> GPTGEAVERAIARVADTIGSGPVNSESIPALTAAETGHTSQVVPADTMQTRHVKNYHSRSESTVENFLCRSACVFYTTYRNHGTDGDNFGYWVISTRQVAQLRRKLEMFTYARFDLELTFVITSTQEQSTIQGQDSPVLTHQIMYVPPGGPVPTKVNSYSWQTSTNPSVFWTEGSAPPRMSIPFISIGNAYSMFYDGWAKFDKQGTYGINTLNNMGTLYMRHVNDGSPGPIVSTVRIYFKPKHVKTWVPRPPRLCQYQKAGNVNFEPTGVTESRTDITTMQTT;> SPSAEECGYSDRVRSITLGNSTITTQECANVVVGYGVWPTYLNDDEATAEDQPTQPDVATCRFYTLESVMWQQSSPGWWWKFPDALSNMGLFGQNMQYHYLGRAGYTVHVQCNASKFHQGCLLVVCVPEAEMGCATLANKPDQKSLSNGETANMFESQNSTGQTAVQANVINAGMGVGVGNLTIFPHQWINLRTNNSATIVMPYINSVPMDNMFRHNNFTLMIIPFAPLSYSTGATTYVPITVTVAPMCAEYNGLRLAGKQ;> GLPTMLTPGSNQFLTSDDFQSPSAMPQFDVTPEMDIPGQVNNLMEIAEVDSVVPVNNTEGKVLSIESYQIPVQSNSTNGSQVFGFPLMPGASSVLNRTLLGEILNYYTHWSGSIKLTFMFCGSAMATGKFLLAYSPPGAGAPTTRKEAMLGTHVIWDVGLQSSCVLCIPWISQTHYRYVVVDEYTAGGYITCWYQTNIVVPADTQSDCKILCFVSACNDFSVRMLKDTPFIKQDNFYQ;> GAQVSTQKTGAHETGLSASGNSIIHYTNVNYYKDAASNSANRQDFTQDPGKFTEPVKDIMIKSMPALN

The genus Enterovirus within the Picornaviridae, a family of non-enveloped viruses with a positive single-stranded RNA genome, is comprised of more than 100 serotypes. Human enteroviruses (EV) are presently classified into four groups, Enterovirus A-D (EV-A, B, C, and D), among which EV-B, the largest group, consists of over 60 serotypes, including all 6 serotypes of coxsackievirus B (CVB1-6), coxsackievirus A9 (CVA9), over 30 serotypes of echoviruses and more than 20 newly identified enteroviruses. The capsid proteins (VP1, VP2, and VP3) adopt the classical eight-stranded anti-parallel β-barrel configuration with the N-termini residing inside and the C-termini exposed on the surface. Most of the uncoating receptors bind to the “canyon” sites of the viral particle, dislodging the “pocket factor” in VP1 and subsequently triggering conformational changes of the intact particle to release the genome, albeit that SCARB2 binds EV71 outside the canyon.

Given that three key structural elements of the VP1 GH, VP2 EF, and VP1 EF loops dominate virus–receptor interactions, we systematically calculated pairwise Euclidean distances between all amino acids for all possible (n2) pairs of these three key elements from 15 structure-available human EVs, which defines a k (k = (n2)) dimensional space delineating the structural characteristics of the receptor-recognition sites. The phylogenetic tree could clearly separate these human EVs into three groups: EV-A, EV-B, and EV-C. Within each group, viruses with distinct receptors were further grouped into mono-phylogenetic clades. This structure-based in silico analysis completely matches the results of experimentally derived receptor identification, therefore, it can be used to deduce the receptor usage for human EVs. To test the robustness of our structure-based algorithm, we determined the structures of three other human EVs (CVB1, CVB5 and Echovirus 3) and put these into our algorithm. The in silico analysis suggests that CVB1 and CVB5 are CAR-dependent human EVs and E3 utilizes FcRn as a functional receptor, predictions consistent with experimental reports.> VANPEHYIKHPLQNRWALWFFKNDKSKTWQANLRLISKFDTVEDFWALYNHIQLSSNLMPG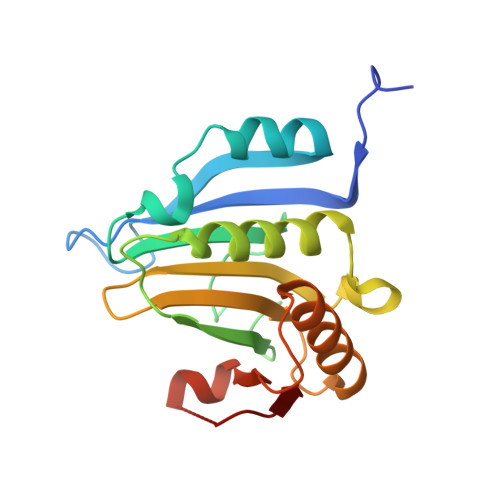CDYSLFKDGIEPMWEDEKNKRGGRWLITLNKQQRRSDLDRFWLETLLCLIGESFDDYSDDVCGAVVNVRAKGDKIAIWTTECENRDAVTHIGRVYKERLGLPPKIVIGYQSHADTATKSGSTTKNRFVV> MRSDGRKEDQLRPVSIQRDFLEYPEGSCLISFGKTKVICTASVIENVPNWLKGKGQGWITAEYSMLPRATQQRTIRESVQGRIGGATHEIQRMIGRAMRTAVELTKIGERTIWVDCDVIQADGGTRTAAITGAFVAVADAIIKLHKEGIIEETPIKDFVAAVSVGIVNDRILLDLNFEEDSAAQVDMNVVGTGSGRLSEVHTMGEEYSFTKDELIKMLDLAQKGINEL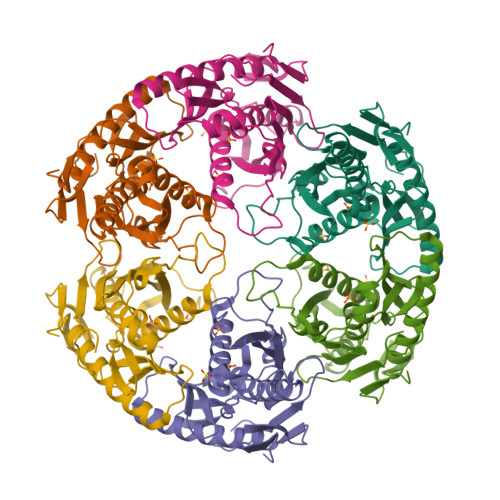IELQKKLYVIQDGKWERSELKEVSSTT RNRs produce all four deoxyribonucleotides and are the only enzymes providing de novo building blocks for DNA replication and repair in all free-living organisms. Class III RNRs, which only function anaerobically, are dimers of an α subunit (NrdD) with a stable radical close to the active site, and binding sites for allosteric nucleotides. Binding of ATP activates RNR, and binding of dATP inhibits it. Here, we present structural, biochemical, and biophysical studies on the ATP-cone-containing NrdD from the human pathogen Prevotella copri (PcNrdD; Nii et al., 2023), showing that the binding of dATP causes increased flexibility of the C-terminal glycyl radical-bearing domain, as well as a flap-like loop that binds across the top of the active site in the active form.

To investigate whether substrate had any allosteric effect on the conformations of the ATP-cone, flap, and GRD, we determined separate cryo-EM structures of tetrameric and dimeric PcNrdD, from the same grid, in the presence of 0.5 mM dATP and 0.5 mM CTP, achieving a resolution of 2.6 Å from 1,105,348 particles before post-processing for the tetramer and 2.6 Å from 1,132,695 particles for the dimer. Both forms were almost identical to those seen in the presence of dATP alone, and no CTP could be seen bound to the active site. Two dATP molecules are bound to each ATP-cone and one at each of the specificity sites, giving a total of 12 visible dATPs per tetramer. The tetramer reveals an arrangement of two dimers (chains A/B and C/D, respectively) in which the ATP-cones are all well-ordered and one ATP-cone from each pair mediates interactions between the dimers. Interestingly, all contacts between the two dimers of the tetramer are mediated by interactions between one of the ATP-cones in one dimer (B or D) and one of the core domains of the other dimer (C or A, respectively). In both forms, the C-terminal GRD is highly mobile in all monomers such that it cannot be seen in the cryo-EM reconstructions. While this allowed us to build complete models for the ATP-cones and analyse dATP binding, the role of tetramerisation in the inhibition mechanism is unclear.

>[4x]GPGSMIQTVVKRDGRIVGFNEQKIMAAIRKAMLHTDKGEDTTLIEQITDHISYRGKSQMSVEAIQDAIEMELMKSARKDVAQKYIAYRNQRNIARKAKTRDVFMSIVNAKNNDITRENANMNADTPAGMMMKFASETTKPFVDDYLLSEDVRDAVMHNYIHIHDKDYYPTKSLTCVQHPLDVILNHGFTAGHGSSRPAKRIETAAVLACISLETCQNEMHGGQAIPAFDFYLAPYVRMSYQEEVKNLEKLTGEDLSNLYDAPIDDYIEKPLDGLQGRERLEQHAINKTVNRVHQAMEAFIHNMNTIHSRGGNQVVFSSINYGTDTSAEGRCIMREILQSTYQGVGNGETAIFPIQIWKKKRGVNYLPEDRNYDLYKLACKVTARRFFPNFLNLDATFNQNEKWRADDPERYKWEIATMGCRTRVFEDRWGEKTSIARGNLSFSTINIVKLAIECMGIENEKQRIDMFFAKLDNILDITAKQLDERFQFQKTAMAKQFPLLMKYLWVGAENLKPEETIESVINHGTLGIGFIGLAECLVALIGKHHGESEKAQELGLKIITYMRDRANEFSEQYHHNYSILATPAEGLSGKFTKKDRKQFGVIPGVTDRDYYTNSNHVPVYYKCTALKKAQIEAPYHDLTRGGHIFYVEIDGDATHNPSVIESVVDMMDKYNMGYGSVNHNRNRCLDCGYENADAHLEVCPKCGSHHIDKLQRITGYLVGTTDRWNSGKLAELHDRVTHIGGEK> KYKKALKKL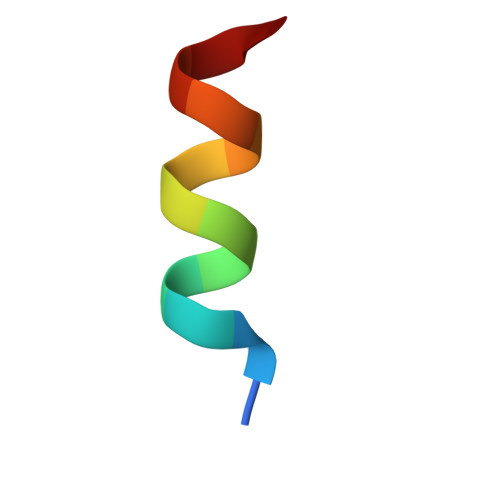AKLL>[4x]MSHVSLQEFLKTEPDGTLEVVAEQYNTTLLEVVRNLPSSTVVPGDKFDTVWDTVCEWGNVTTLVHTADVILEFSGELPSGFHRHGYFNLRGKHGMSGHIKAENCTHIALIERKFMGMDTA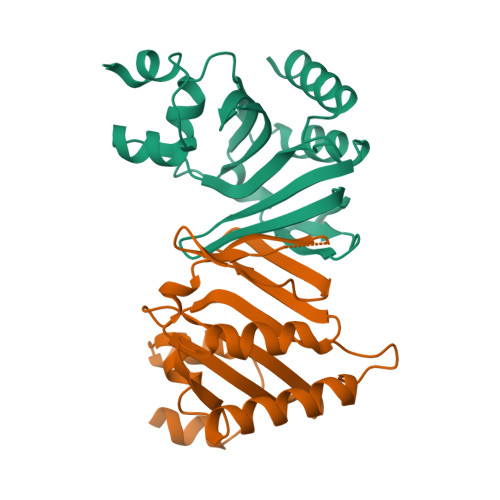SILFFNKEGSAMLKIFLGRDDHRQLLSEQVSAFHTLAASLKEHA> SNAASGGRALRVLVDMDGVLADFEGGFLRKFRARFPDQPFIALEDRRGFWVSEQYGRLRPGLSEKAISIWESKNFFFELEPLPGAVEAVKEMASLQNTDVFICTSPIKMFKYCPYEKYAWVEKYFGPDFLEQIVLTRDKTVVSADLLIDDRPDITGAEPTPSWEHVLFTACHNQHLQLQPPRRRLHSWAD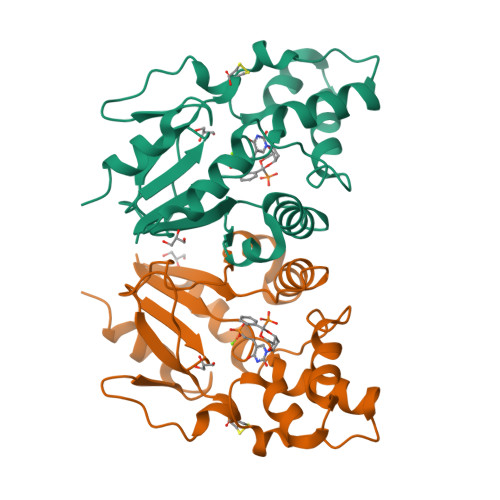DWKAILDSKRPC> AWPAWPAWPAWP;> KKEAEEVAAHVEQIAFI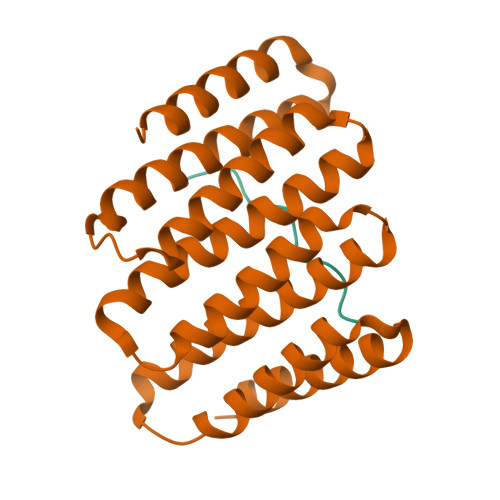AKEQGNEEVAKLAKRLAETIKRLNEGTEEEVKRLLEAAEVAAHVLQIAFIAHEQGNEEVAKLALELAESILRLIEGTEEEVKRLLEAAEVAAHVLQIAFIAHEQGNEEVAKLALELAESILRLIEGTEEEVKELLERAEEAAHVLQHAFIATEQGNEEDAKEALRKAEEILRRNA>EAEAADRADILYNIRQTSRPDVIPTQRDRPVAVSVSLKFINILEVNEITNEVDVVFWQRTTWSDRTLAWDSSHSPDQVSVPISSLWVPDLAAYNAISKPEVLTPQLARVVSDGEVLYMPSI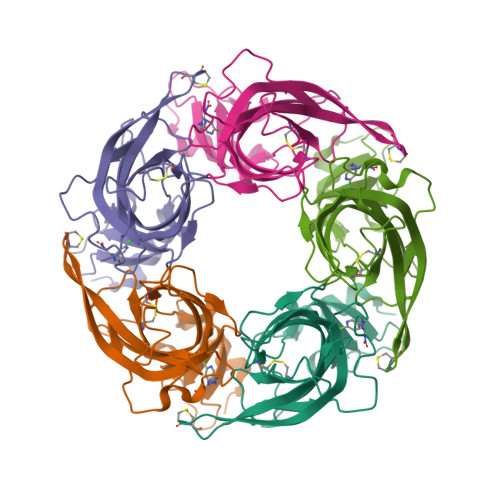RQRFSCDVSGVDTESGATCRIKIGSWTHHSREISVDPTTENSDDSEYFSQYSRFEILDVTQKKNSVTYSCCPEAYEDVEVSLNFRKKGRSEIL[5x]> MAHHHHHHVGTGSNDDDDKSPDPWELTILHTNDVHSRLEQTSEDSSKCVDASRCMGGVARLFTKVQQIRRAEPNVLLLDAGDQYQGTIWFTVYKGAEVAHFMNALRYDAMALGNHEFDNGVEGLIEPLLKEAKFPILSANISASGPLASQISGLYLPYKVLPVGDEVVGIVGYTSKETPFLSNPGTNLVFEDEITALQPEVDKLKTLNVNKIIALGHSGFEMDKLIAQKVRGVDVVVGGHSNTFLYTGNPPSKEVPAGKYPFIVTSDDGRKVPVVQAYAFGKYLGYLKIEFDERGNVISSHGNPILLDSSIPEDPSIKADINKWRIKLDDYSTQELGKTIVYLDGSSQSC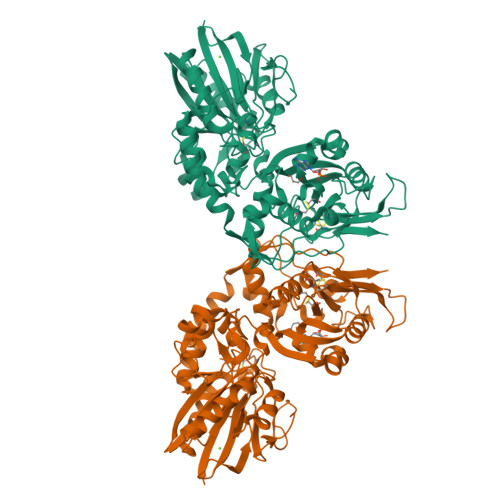RFRECNMGNLICDAMINNNLRHADEMFWNHVSMCILNGGGIRSPIDERNDGTITWENLAAVLPFGGTFDLVQLKGSTLKKAFEHSVHRYGQSTGEFLQVGGIHVVYDLSRKPGDRVVKLDVLCTSCRVPSYDPLKMDEVYKVILPNFLANGGDGFQMIKDELLRHDSGDQDINVVSTYISKMKVIYPAVEGRIKFS>[2x]MQTTANHSSRSTQTGTRAHGAALAETTSREDFRALATEHRVVPVIRKVLADSETPLSAYRKLAANRPGTFLLESAENGRSWSRWSFIGAGAPSALTVRDNAAAWLGTAPEGAPSGGDPLDALRATLDLLKTEAMAGLPPLSSGLVGFFAYDMVRRLERLPELAVDDLGLPDMLLLLATDIAAVDHHEGTITLIANAVNWNGTDERVDWAYDDAVARLDVMTKALGQPLTSAVATFSRPAPDHRAQRTMEEYTEIVDKLVGDIEAGEAFQVVPSQRFEMDTAADPLDVYRILRVTNPSPYMYLLNIPDADGGLDFSIVGSSPEALVTVKDGRATTHPIAGTRWRGATEEEDVLLEKELLADEKERAEHLMLVDLGRNDLGRVCRPGTVRVDDYSHIERYSHVMHLVSTVTGELAEDKTALDAVTACFPAGTLSGAPKVRAMELIEEVEKTRRGLYGGVVGYLDFAGNADFAIAIRTALMRNGTAYVQAGGGVVADSNGPYEYTEA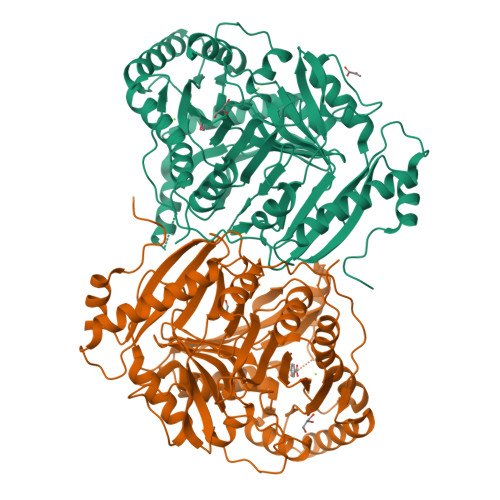ANKARAVLNAIAAAATLAEP In summary, our study demonstrates that PH0208 protein would function as a purine nucleotide dependent R15Pi enzyme and not as a homologue of the regulatory subunit of eIF2B. In NMP degradation pathway, R15Pi catalyzes the conversion of ribose-1,5-bisphosphate (R15P, substrate) into ribulose-1,5-bisphosphate (RuBP, product) in an adenosine 5′-monophosphate (AMP)-dependent manner. AMP acts as an activator of R15Pi and in its absence the enzymatic activity has been found to decline dramatically. Monomer of PH0208 protein consists of an N-terminal α-helical domain (residues 1–122) and a C-terminal α-β-α sandwich domain (residues 123–324).

To verify the preferred molecule at the ‘AMP binding site’, PH0208-WT, PH0208-C135S and PH0208-D204N were crystallized in the presence of both AMP and GMP. In the presence of both the potential ligands, AMP outcompete GMP and binds to the ‘AMP binding site’ utilizing the similar set of amino acid while GMP binds to the ‘GMP binding loop’. During crystallization, even a higher concentration of GMP (4.5 mM) as compared to AMP (1.5 mM) could not aid GMP to occupy the ‘AMP binding site’. This further indicates a higher affinity of AMP at the ‘AMP binding site’. Evidently, when both AMP and GMP were made available, AMP binds to the ‘AMP binding site’ with a higher preference than GMP, while GMP occupies the ‘GMP binding loop’ only. Binding of GMP to the ‘GMP binding loop’ involves very few interactions which predominantly includes only the guanosine base ring of the GMP molecule. Thus, it might also be possible that the binding of GMP to the ‘GMP binding loop’ is an outcome of crystallization artifact. Both, AMP and GMP bind to PH0208 protein even after the mutation of the catalytic residues (PH0208-C135S and PH0208-D204N) at the active site pocket.

>MGAMIVKEVYETAEKIKSMEIRGAGRIARAAAQALMIQAEKSKAKEPEELWNELKVASKILYNTRPTAVSLPNALRYVMHRVKAAYLGGADLETLRFTAINSAKEFIYNSEKAIERIGEIGAKRIEDGDIIMTHSHSKAAISVMKKAFEQGKNIKVIVTETRPKWQGKITAKELASYGIPVIYIVDSAARHYMKMTDKVVMGADSITANGAVINKIGTSLIALTAKEHRVWVMIAAETYKFHPATMLGQLVEIEMRDPTEVIPEEELRTWPKNIEVWNPAFDVTPPEYIDVIITERGIIPPYAAIDILKEEFGWALKYKEPWED[3x]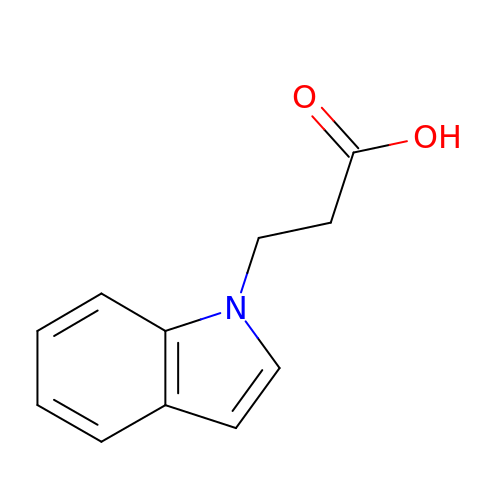3-indol-1-ylpropanoic acid | C11 H11 N O2 | OSWNOVFZARRSKM-UHFFFAOYSA-N>MVEATAQETDRPRFSFSIAAREGKARTGTIEMKRGVIRTPAFMPVGTAATVKALKPETVRATGADIILGNTYHLMLRPGAERIAKLGGLHSFMGWDRPILTDSGGYQVMSLSSLTKQSEEGVTFKSHLDGSRHMLSPERSIEIQHLLGSDIVMAFDECTPYPATPSRAASSMERSMRWAKRSRDAFDSRKEQAENAALFGIQQGSVFENLRQQSADALAEIGFDGYAVGGLAVGEGQDEMFRVLDFSVPMLPDDKPHYLMGVGKPDDIVGAVERGIDMFDCVLPTRSGRNGQAFTWDGPINIRNARFSEDLKP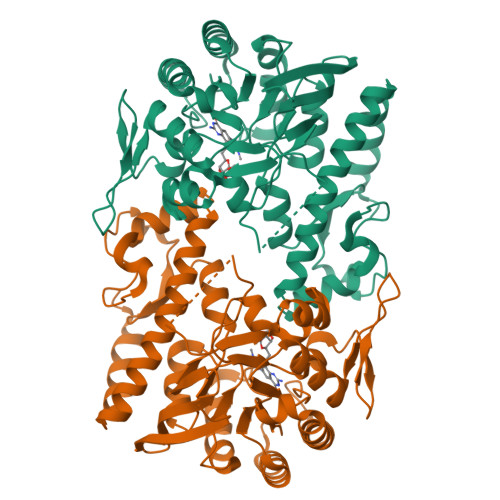LDSECHCAVCQKWSRAYIHHLIRAGEILGAMLMTEHNIAFYQQLMQKIRDSISEGRFSQFAQDFRARYFARNS[2x]> XVE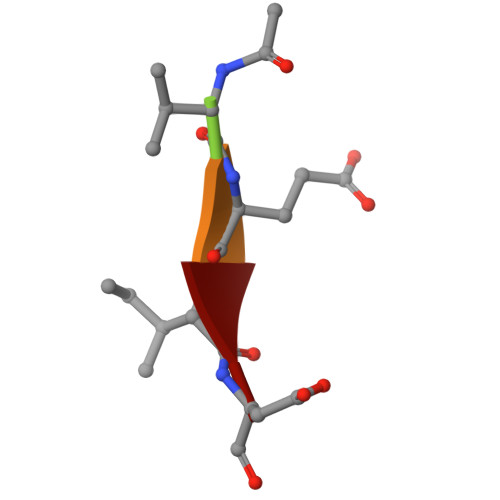ID>MMLSLNNLQNIIYNPVIPFVGTIPDQLDPGTLIVIRGHVPSDADRFQVDLQNGSSMKPRADVAFHFNPRFKRAGCIVCNTLINEKWGREEITYDTPFKREKSFEI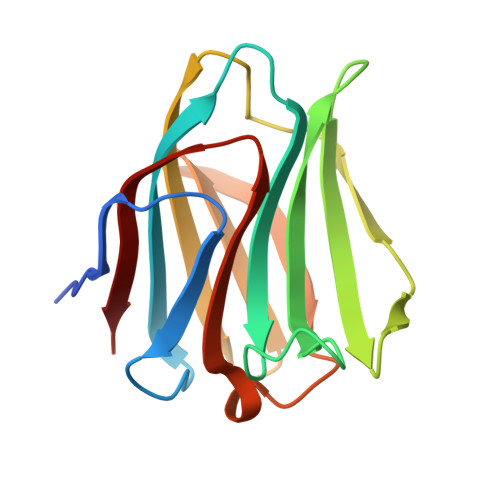VIMVLKDKFQVAVNGKHTLLYGHRIGPEKIDTLGIYGKVNIHSIGFSF[2x]>[4x]GACCGUCAAAUUGC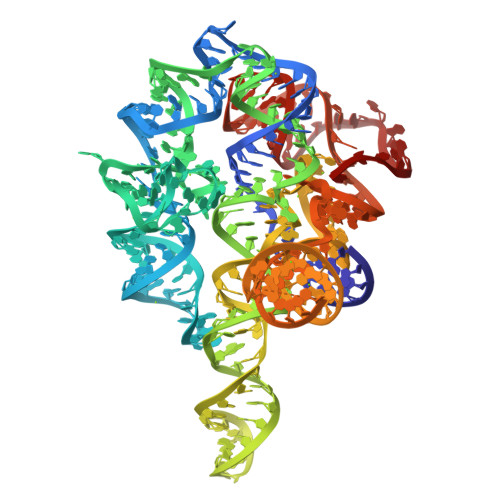GGGAAAGGGGUCAACAGCCGUUCAGUACCAAGUCUCAGGGGAAACUUUGAGAUGGCCUUGCAAAGGGUAUGGUAAUAAGCUGACGGACAUGGUCCUAACCGCGCAGCCAAGUCCUAAGUCAACAGGAGACUGUUGAUAUGGAUGCAGUACACAGACUAGAUGUCGGCCGGGGAAGAUGUAUUCUUCUCAUAAGGUAUAGUCGGACCUCUCCCGAAAGGGAGUUGGAGUACUCG> HSNEKWFHGKLGAGRDGRHIAERLLTEYCIETGAPDGSFLVRESETFVGDYTLSFWRNGKVQHCRIHSRQDAGTPKFFLTDNLVFDSLYDLITHYQQVPLRCNEFEMRLSEPVPQTNAHESKEWYHASLTRAQAEHMLMRVPRDGAFLVRKRNEPNSYAIS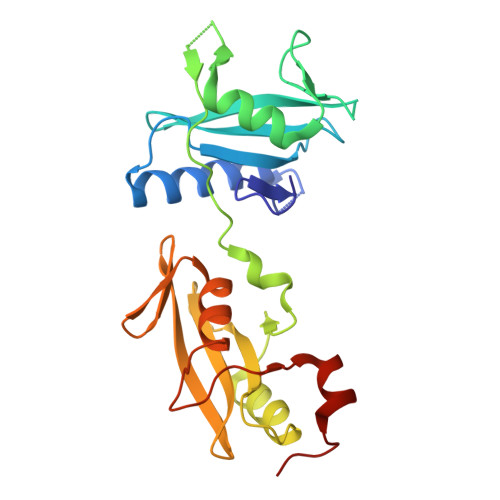FRAEGKIKHCRVQQEGQTVMLGNSEFDSLVDLISYYEKHPLYRKMKLRYPINEEALEKIGTAEPDYG> LAKRIIACLDVKDGRVVKPTNFENLRDSGDPVELGKFYSEIGIDELVFLDITASVEKRKTMLELVEKVAEQIDIPFTVGGGIHDFETASELIL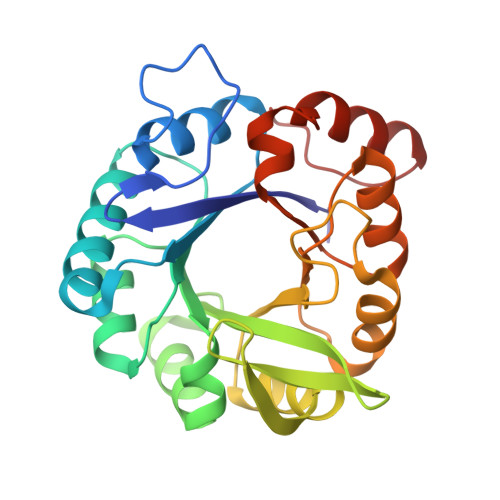RGADKVSINTAAVENPSLITQIAQTFGSQAVVVAIDAKRVDGEFMVFTYSGKKNTGILLRDWVVEVEKRGAGEILLTSIDRDGTKSGYDTEMIRFVRPLTTLPIIASGGAGKMEHFLEAFLAGADAALAASVFHFREIDVRELKEYLKKHGVNVRLEL>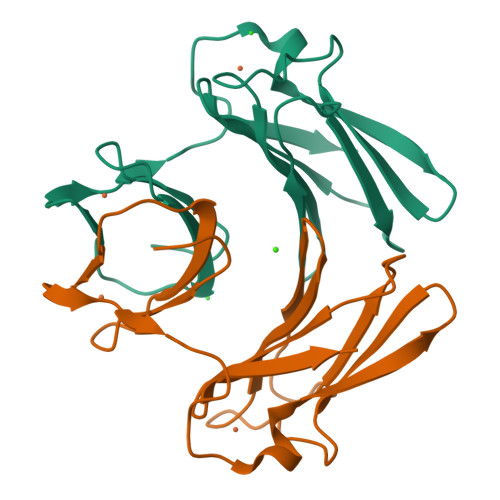MPERLQVYKCEVCGNIVEVLNGGIGELVCCNQDMKLMSENTVDAAKAKHVPVIEKIDGGYKVKVGAVAHPMEEKHYIQWIELLADDKCYTQFLKPGQAPEAVFLIEAAKVVAREYCNIHGHWKAEN[2x]5-methyl-N-(1-methyl-1H-pyrazol-4-yl)-1,2-oxazole-3-carboxamide 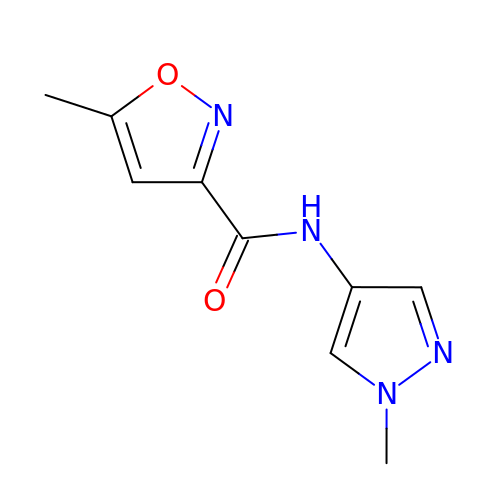| C9 H10 N4 O2 | NZGVYOGTUDYUSZ-UHFFFAOYSA-N>LPNITILATGGTIAGGGDSATKSNYTAGKVGVENLVNAVPQLKDIANVKGEQVVNIGSQDMNDDVWLTLAKKINTDCDKTDGFVITHGTDTMEETAYFLDLTVKCDKPVVMVGAMRPSTSMSADGPFNLYNAVVTAADKASANRGVLVVMNDTVLDGRDVTKTNTTDVATFKSVNYGPLGYIHNGKIDYQRTPARKHTSDTPFDVSKLNELPKVGIVYNYANASDLPAKALVDAGYDGIVSAGVGNGNLYKTVFDTLATAAKNGTAVVRSSRVPTGATTQDAEVDDAKYGFVASGTLNPQKARVLLQLALTQTKDPQQIQQIFNQY[2x]

l-asparaginase II (EC 3.5.1.1) is an amidohydrolase that primarily catalyzes the hydrolysis of l-Asn to l-Asp and ammonia, but that can also act on other substrates, including l-Gln. This enzyme has been used for over 40 years in the treatment of leukemias, particularly Acute Lymphoblastic Leukemia (ALL), which is the most prevalent cancer in childhood. Many studies focus on the EcA2 from the K12 strain (EcA2-K12), which differs by four amino acids from reference biopharmaceuticals, including Elspar (EcA2-4M). To understand the structural implications of the four-amino acid differences between EcA2-K12 and EcA2-4M, we solved their crystal structure in the presence of l-Asp under the same crystallization condition and data collection method.

The most prevalent amino acid sequence observed in EcA2 biopharmaceuticals, including pegylated forms such as Pegaspargase and Calaspargase, as well as the reference product Elspar, differs from that of the K12 strain by four amino acid substitutionsV27A, N64D, S252T, and T263Nand is referred to here as EcA2-4M. This EcA2-4M sequence corresponds to asparaginase from other strains, including BL21­(DE3) (GenBank: CAQ33267; ACN38272.1). The EcA2 from BL21­(DE3), hereby cited as EcA2-4M, is the prevalent form used in commercial pharmaceutical preparations of l-asparaginase, including Elspar (the innovator product, approved by the FDA in 1978), Spectrila, and their PEGylated versions, respectively Oncaspar and Asparlas. All monomers in the asymmetric unit showed the l-Asp in the active site. The monomers of EcA2-K12 and EcA2-4M were essentially superposable, with Cα RMSD values lower than 0.4 Å. The specific activity of EcA2-K12 and EcA2-4 M was assessed by monitoring the hydrolysis of the l-Asn in vitro. These results demonstrate that the EcA2-4 M variant exhibits approximately twice the specific activity of EcA2-K12, with values of 69 ± 4 and 25 ± 2 IU/mg, respectively. However, the results show that the EcA2-4 M variant exhibits a substrate turnover rate (k cat) approximately twice that of EcA2-K12, which can explain the differences in specific activity and cytotoxicity. The analysis of the binding curves obtained from this experiment allowed for the calculation of the dissociation constant (K D) of the enzymes for l-Asp. This analysis demonstrated that the EcA2-K12 variant has a dissociation constant for the product of the catalyzed reaction that is three times higher than that of the EcA2-4M variant, with K D values of 211 ± 52 and 66 ± 14 μM, respectively. The titration with l-Asp indicates that the EcA2 4 M variant requires a lower concentration of ligand, 100–150 μM, for the stabilization of its closed form, evidenced by the disappearance of the Hε and Hδ signals from the aromatic ring of Tyr25. In contrast, the EcA2-4M variant shows lower specificity for l-Asn, with a k cat Asn/k cat Gln ratio of 18.2 ± 0.2.2,4-bisacetamido-2,4,6-trideoxy-beta-D-glucopyranose | C10 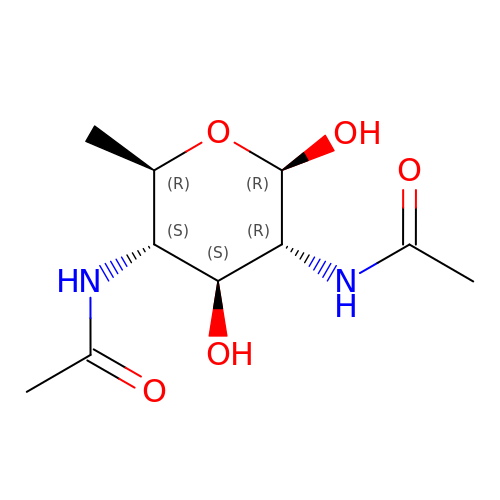H18 N2 O5 | NRXWTRNYICXMBF-DAJIKZSHSA-N> GAMDKQKPRYEIRWRVIESISPDGHEYIYVDPMQLPYDSRWEFPRDGLVLGRVLGSGAFGKVVEGTAYGLSRSQPVMKVAVKMLKPTARSSEKQALMSELKIMTHLGPHLNIVNLLGACTKSGPIYIIIEYCFYGDLVNYLHKNRDSFLSHKKKSMLDSEVKNLLSDDNSEGLTLLDLLSFTYQVARGMEFLASKNCVHRDLAARNVLLAQGKIVKICDFGLARDIMHDSNYVSKGSTFLPVKWMAPESIFDNLYTTLSDVWSYGILLWEIFSLGGTPYPGM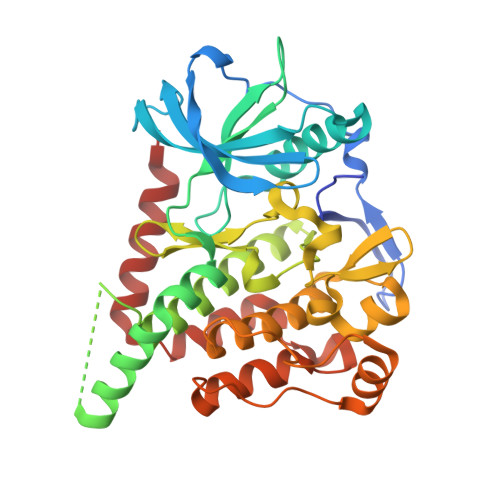MVDSTFYNKIKSGYRMAKPDHATSEVYEIMVKCWNSEPEKRPSFYHLSEIVENLLPGQYKKSYEKIHLDFLKSD(3E,7aR,12aS)-3-[(1H-imidazol-4-yl)methylidene]-6,12-dimethoxy-7a-(2-methylbut-3-en-2-yl)-7a,12-dihydro-1H,5H-imidazo[1',2':1,2]pyrido[2,3-b]indole-2,5(3H)-dione 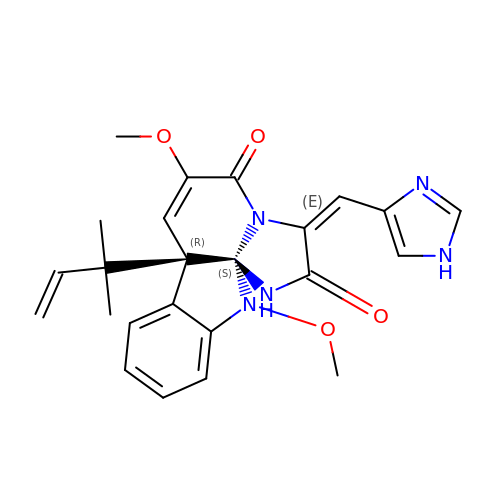| C24 H25 N5 O4 | SOHAVULMGIITDH-ZXPSTKSJSA-N D-ALLOSE | C6 H12 O6 | 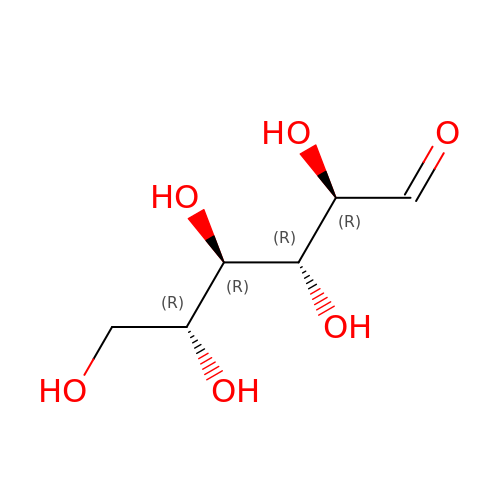GZCGUPFRVQAUEE-BGPJRJDNSA-N>[4x]MALVDGFLELERSSGKLEWSAILQKMASDLGFSKILFGLLPKDSQDYENAFIVGNYPAAWREHYDRAGYARVDPTVSHCTQSVLPIFWEPSIYQTRKQHEFFEEASAAGLVYG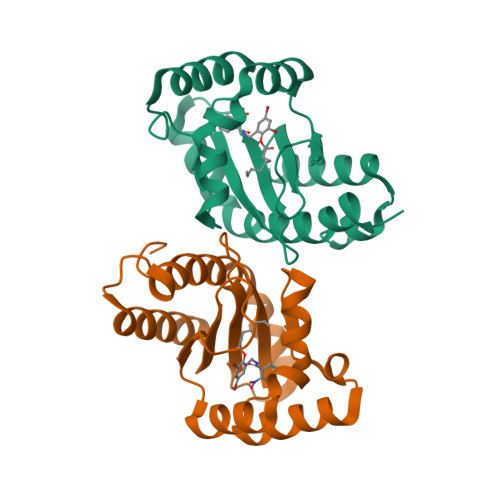LTMPLHGARGELGALSLSVEAENRAEANRFMESVLPTLWMLKDYALQSGAGLAFEHP>MGSSHHHHHHSSGLVPRGSHSQPSTANGGFPSVVVTAVTATTSISPDIESTWKGLLAGESGIHALEDEFVTKWDLAVKIGGHLKDPVDSHMGRLDMRRMSYVQRMGKLLGGQLWESAGSPEVDPDRFAVVVGTGLGGAERIVESYDLMNAGGPRKVSPLAVQMIMPNGAAAVIGLQLGARAGVMTPVSACSSGSEAIAHAWRQIVMGDADVAVCGGVEGPIEALPIAAFSMMRAMSTRNDEPERASRPFDKDRDGFVFGEAGALMLIETEEHAKARGAKPLARLLGAGITSDAFHMVAPAADGVRAGRAMTRSLELAGLSPADIDHVNAHGTATPIGDAAEANAIRVAGCDQAAVYAPKSALGHSIGAVGALESVLTVLTLRDGVIPPTLNYETPDPEIDLDVVAGEPRYGDYRYAVNNSFGFGGHNVALAFGRY[2x]

In addition, through MoA studies, we identify the M. tuberculosis cellular target of GSK3011724A to be KasA, a β-ketoacyl synthase. Mycolic acids are unique and fundamental components of the mycobacterial cell wall and KasA is essential in M. tuberculosis. The FAS-II system is comprised of four enzymes acting in a consecutive cycle: KasA and KasB, condensing enzymes; MabA, a keto-reductase34; HadABC, a dehydratase35; and InhA, an enoyl-reductase36. The FAS-II system enables fatty acid elongation leading to meromycolic acids (C56), which are then condensed with C26-CoA (from FAS-I) by the polyketide synthase Pks13, followed by reduction, culminating in the production of mature mycolic acids.

Curious to understand the molecular details of GSK3011724A binding to KasA, a 2.13 Å co-crystal structure of the dimeric KasA-GSK3011724A complex was solved. The co-crystal structure reveals that, in contrast to TLM, GSK3011724A uniquely binds within the large acyl channel that normally accommodates the growing meromycolic acid chain, unexpectedly trapping the open conformation of the enzyme. GSK3011724A sits at the branch point of the acyl channel, a feature thought to confer specificity for ‘kinked' unsaturated substrates. Within this site, density for a long linear molecule, modelled as polyethylene glycol (PEG), is also consistently present and perfectly complements the space between the compound and the protein. This sandwich of PEG and GSK3011724A enables the large acyl cavity to be filled, occupying the volume of the branched phospholipid chains previously observed within this pocket. The indazole ring lies across the flat hydrophobic surface formed by residues such as Gly200 and Pro201, and the amide of the sulfonamide makes a key hydrogen bond with Glu199. This anchors the ligand in an ideal position, allowing the kink (introduced by the sulfonamide linkage) to place the butyl chain into an orthogonal narrow lipophilic channel lined by residues such as Ile347, Ile202 and Phe239. Pro201 and Pro206 both lie within the acyl site and are in direct contact with the ligand. Exchange of proline for a hydrophilic serine residue (Pro201Ser) disfavours interactions with the aromatic indazole ring, whereas the Pro206Leu substitution introduces steric crowding of the ligand. An explanation of this finding comes from close inspection of the GSK3011724A-KasA complex crystal structure, where specific changes in the acyl pockets of the related enzymes disfavour the unique binding mode of GSK3011724A.>HGSYIDITIDLKHYNGSVFDLRLSDYHP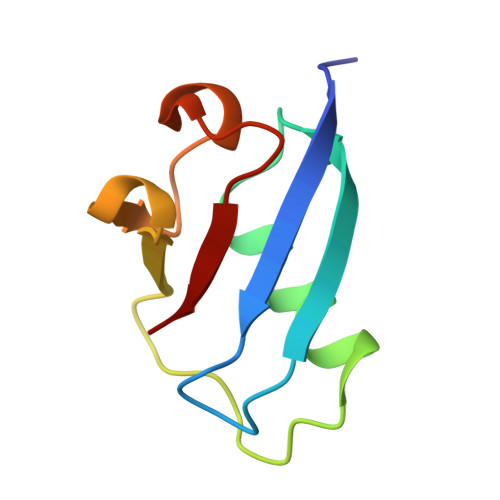VKKVIDIAWQAQSVSMPPREGHWIRVVNKDKVFSGECKLSDCGITNGDRLEIL[2x]1-AMINO-2,3-DIHYDROXY-5-HYDROXYMETHYL CYCLOHEX-5-ENE | C7 H13 N O3 | 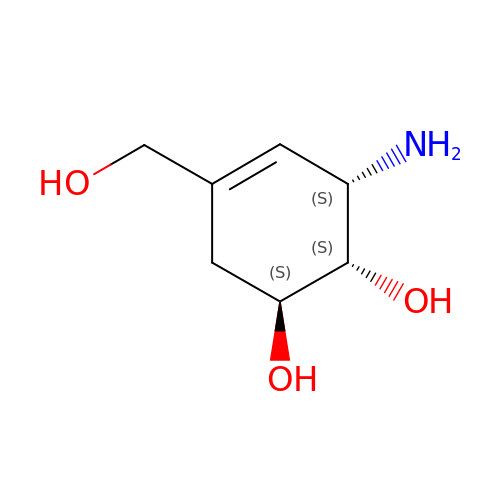BMZJPVSGERKRHP-ACZMJKKPSA-N>HPETLVKVKDAEDQLGARVGYIELDLNSGKILESFRPEERFPMMSTFKVLLCGAVLSRVDAGQEQLGRRIHYSQNDLVEYSPVTEKHLTDGMTVRELCSAAITMSDNTAANLLLTTIGGPKELTAFLHNMGDHVTRLDRWEPELNEAIPNDERDTTMPAAMATTLRKLLTGELLTLASRQQLIDWMEADKVAGPLLRSALPAGWFIADKSGAGERGSRGIIAALGPDGKPSRIVVIYTTGSQATMDERNRQIAEIGASLIK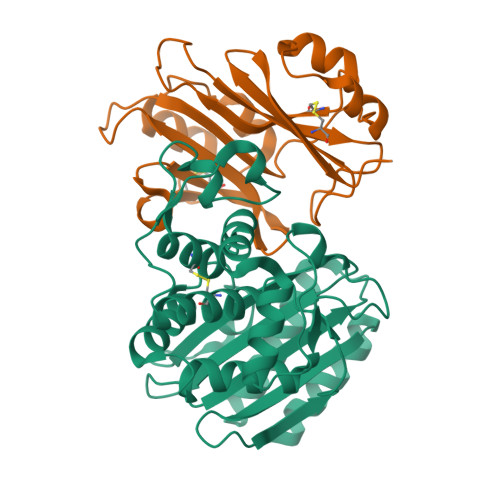HW[2x];>[2x]AGVMTGAKFTQIQFGMTRQQVLDIAGAENCETGGSFGDSIHCRGHAAGDYYAYATFGFTSAAADAKVDSKSQWKLLAPSAPTLTLAKFNQVTVGMTRAQVLATVGQGSCTTWSEYYPAYPSTAGVTLSLSCFDVDGYSSTGFYRGSAHLWFTDGVLQGKRQWDLV> MSSHHHHHHSSAMASTAENLYFQGGITFTVMIVGQSGSGRSTFINTLCGQQVVDTSTTILLPTDTSTEIDLQLREETVELEDDEGVKIQLNIIDTPGFGDSLDNSPSFEIISDYIRHQYDEILLEESRVRRNPRFKDGRVHCCLYLINPTGHGLKEIDVEFIRQLGSLVNIIPVISKSDSLTRDELKLNKKLIMEDIDRWNLPIYNFPFDEDEISDEDYETNMYLRTLLPFAIIGSNEVYEMGGD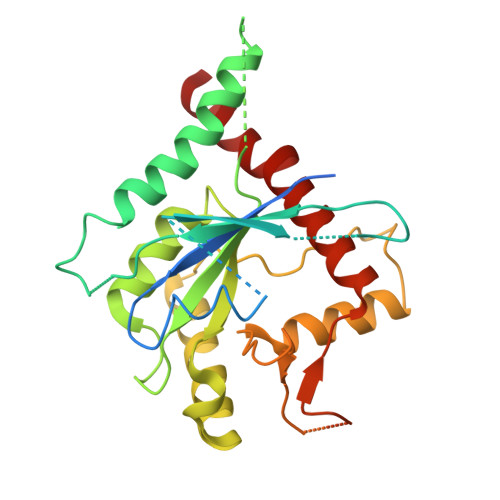VGTIRGRKYPWGILDVEDSSISDFVILRNALLISHLHDLKNYTHEILYERYRTEALSG> GPLGSVWQLISKVLARHFSAADASRVLEQLQRDYERSLSRLTLDDIERLASRFLHPEV;> GPLGSAKRRKTMQGEGPQLLLSEAVSRAAKAAGARPLTSPESLSRDLEAPEVQESYRQQLRSDIQKRLQEDPNYSPQRFPN

BAG6 is an essential protein that functions in two distinct biological pathways, ubiquitin-mediated protein degradation of defective polypeptides and tail-anchored (TA) transmembrane protein biogenesis in mammals, although its structural and functional properties remain unknown. Recent work showed that BAG6 is also a mediator of tail-anchored (TA) transmembrane protein biogenesis. In the TA protein assembly pathway, BAG6 holds the hydrophobic transmembrane domain of newly synthesized TA proteins to maintain them in an unfolded but soluble state in the cytosol. Similarly, mammalian BAG6, Ubl4a, and SGTA make up a trimeric complex that binds TA proteins post-translationally and then loads them onto the cytosolic ATPase TRC40, which in turn targets them to the endoplasmic reticulum.

The x-ray crystal structure of the complex was determined at 1.85 Å resolution. Unambiguous electron density allowed modeling of residues 1058–1112 of BAG6 BAGS and 94–143 of Ubl4a TUGS. The overall structure of the complex consists of six α-helices, three from BAG6 BAGS and three from Ubl4a TUGS. The structure of the first (α1TUGS, residues 95–104) and the second (α2TUGS, residues 109–128) α-helices of Ubl4a TUGS is nearly identical to that of the C-terminal dimerization domain in yeast Get5 (28), despite the extensive divergence in the primary sequences, especially at the protein surfaces. BAG6 BAGS consists of three α-helices, residues 1064–1075 (α1BAGS), 1083–1090 (α2BAGS), and 1093–1112 (α3BAGS). The tertiary structure of BAG6 BAGS was quite distinct from that of the canonical BAG domain identified in BAG1, which adopts a three-helix bundle fold. α1BAGS crosses with α2TUGS forming at a 60° angle, and α2BAGS crosses with α1TUGS forming at a 20° angle, respectively, forming a four-α-helix bundle. The dimer interface primarily consists of the hydrophobic patch on BAG6 (Leu-1064, Val-1068, Ala-1071, and Ala-1072 in α1BAGS; Ala-1077, Pro-1079, and Leu-1080 in the loop region of α1BAGS and α2BAGS; Leu-1086, and Leu-1090 in α2BAGS; and Tyr-1099 in α3BAGS) that docks against Ubl4a (Val-95, Leu-98, Ile-99, and Val-102 in α1TUGS; Phe-107 in the loop region between α1TUGS and α2TUGS; and Val-115, Leu-119, and Tyr-123 in α2TUGS). His-106 of Ubl4a forms electrostatic bridges with Thr-1081 (2.7 Å) and Asp-1089 (2.6 Å) of BAG6, and all of these residues are conserved across vertebrates. One CHAPS molecule was visible in this crystal structure, and it interacted with α3TUGS and α3BAGS.>[4x]SEEMIDHRLTDREWAEEWKHLDHLLNCIMDMVEKTRRSL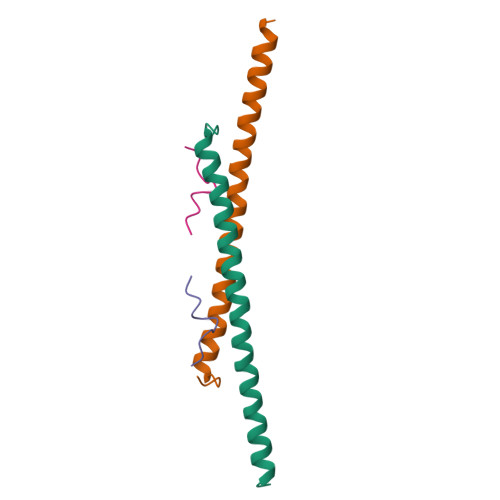TVLRRCQEADREELNYWIRRYSDAE;>SPLQAKKVRKVPPGLPSSVYAPSPN[4x]> GH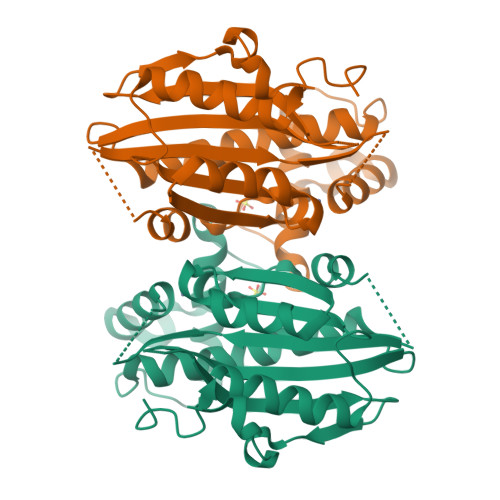MASQALTVSQSKAVAPSNGAPAPLAQVEEVDIARHMNDRHAHILRYFPTALGVDDFMARTEIVLGGFGFTGDNTIAMTNLCRDEVTQVVKDKIEAAFGSSFNTNGLGAVLTCGVTGMKAGLSHSPVCAGGRERYVFFAFPHIAINSEGEVGAISRPGRPKMSCACGALQKCLVELKAEGVDAAVRAPGLHDPIEPEYSILKQRLARRIRYEKLDPQLMDLPSLTALAERTISDDLEYLIEKAVNPATSDYAVITGVEIHNWAAHLEEGGDPSMEFIAPTKAYVVVNGVKTHLDLMMVPPMSFRQLQ> GLPTLSTPGSNQFLTSDDFQSPSAMPQFDVTPEMDI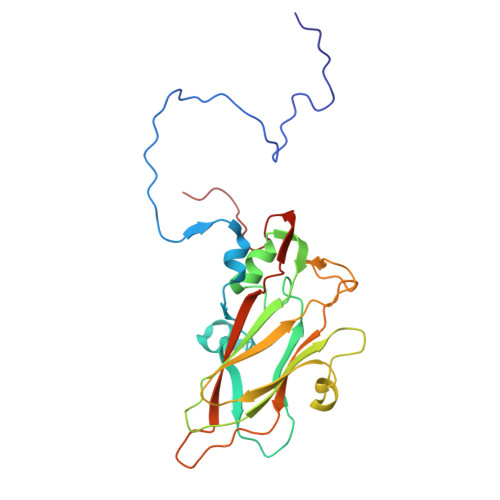PGQVNNLMEIAEVDSVVPVNNTEGKVMSIEAYQIPVQSNPTNGSQVFGFPLTPGANSVLNRTLLGEILNYYAHWSGSIKLTFMFCGSAMATGKFLLAYSPPGAGAPTTRKEAMLGTHVIWDVGLQSSCVLCIPWISQTHYRYVVMDEYTAGGYITCWYQTNIVVPADAQSDCKILCFVSACNDFSVRMLKDTPFIKQDNFFQ> LEQSAARQHAQVDAEQALAQVNARIAELHKMPQAQVPASEAPKVNYGEEIRKLLDTAFELRTAIESIIAGKVPPVDLSTIPARVDLLTTSVKTIQQANHNLVNKVEAAHVELGFSITRALIRTINPTSTAAQLAESKADVLSTYAKVAAYRDLKPTDAATVYVKNRLNTKIWQTRINRDKYLLGKNAEGYKAINKALTHATGVWFNPATTVKQV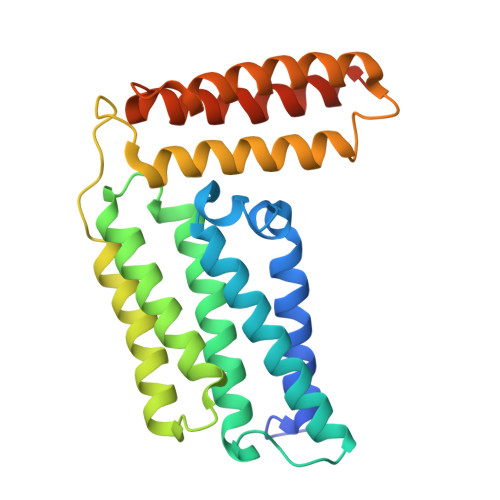DDEVKALDLAFQAALDRRPADGKLRTNAA>[6x]MQQSVCRARPIWWGTQRRGSETMAGAAVKYLSQEEAQAVDQELFNEYQFSVDQLMELAGLSCATAIAKAYPPTSMSKSPPTVLVICGPGNNGGDGLVCARHLKLFGYQPTIYYPKRPNKPLFTGLV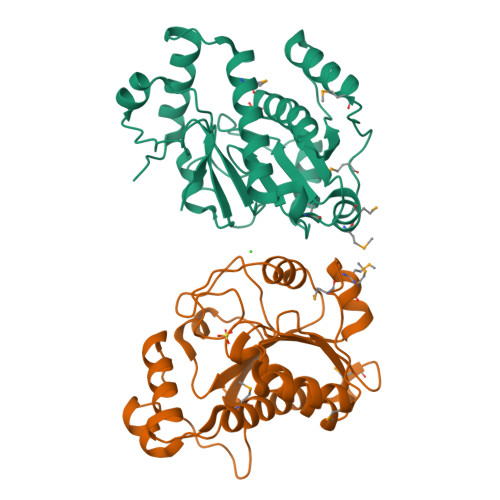TQCQKMDIPFLGEMPPEPMMVDELYELVVDAIFGFSFKGDVREPFHSILSVLSGLTVPIASIDIPSGWDVEKGNPSGIQPDLLISLTAPKKSATHFTGRYHYLGGRFVPPALEKKYQLNLPSYPDTECVYRLQHHHHHH>[4x]MFSDLKGKRILITGSSQGIGMATAIELARYGAVVGLHGRKAPADPALLLGKLREAGGDGAFFRADITKTAECQRLVSAFVERFDGIDVLINNAGGLAGRSNLENIDDAFYDRVMDLNGRSVLMMTKFAIPHLRASAKASGTTSAVISTGSIAAREGGGIG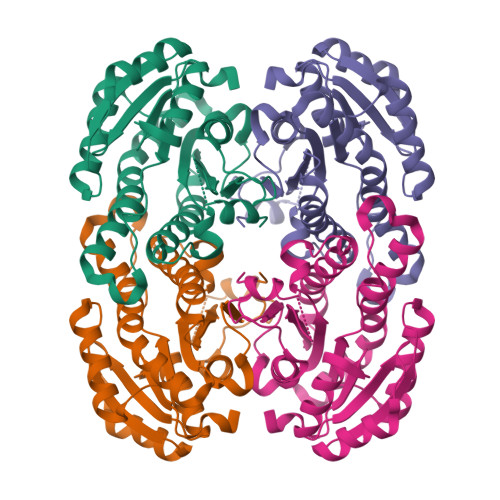AGVYAASKAWLHDIHRNWVKEFTKDSIRFNIVAPGTVDTAFHADKSDELKTRIANSIPMGRFGTVQELAPAYVFFASHAASGYITGQILDVNGGQICP> HRFKVYNYMSPTFC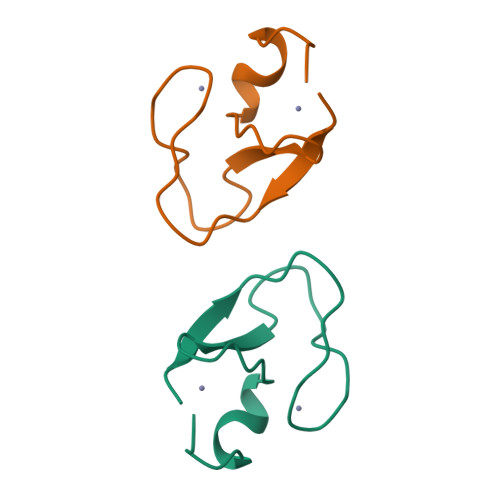DHCGSLLWGLVKQGLKCEDCGMNVHHKCREKVANLC TERT-BUTYL(1S)-1-CYCLOHEXYL-2-OXOETHYLCARBAMATE 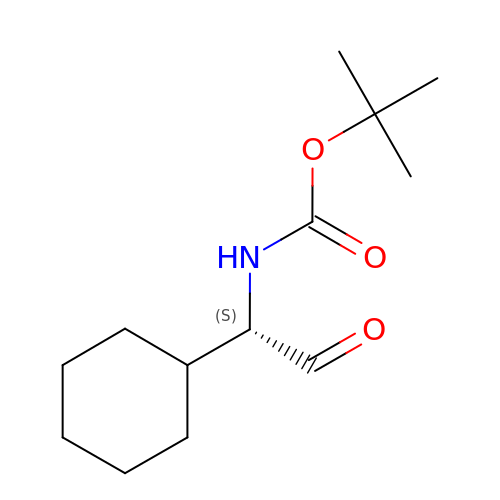| C13 H23 N O3 | BDSGOSWEKUGHOV-LLVKDONJSA-N> GSMSAPDSITVTVADHNG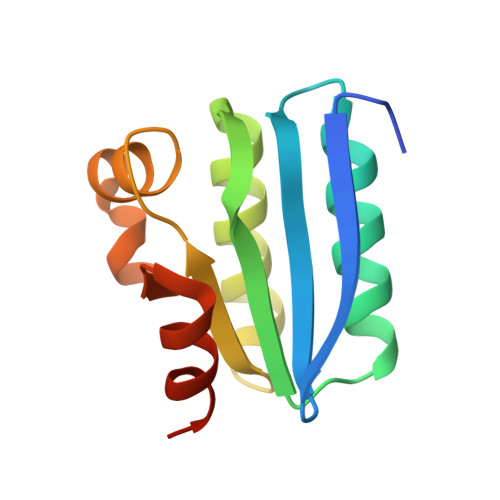VAVLSIGGEIDLITAAALEEAIGEVVADNPTALVIDLSAVEFLGSVGLKILAATSEKIGQSVKFGVVARGSVTRRPIHLMGLDKTFRLFSTLHDALTGVRGGRIDR(2S)-3-amino-2-{[(4-cyclohexylbutoxy)carbonyl]amino}propanethioic 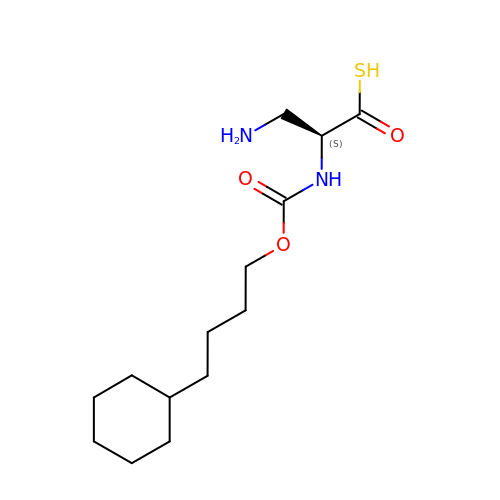S-acid | C14 H26 N2 O3 S | PRQLPRBNQTXHJV-LBPRGKRZSA-N> PISPIETVPVKLKPGMDGPKVKQWPLTEEKIKALVEICTEMEKEGKISKIGPENPYNTPVFAIKKKDSTKWRKLVDFRELNKRTQDFWEVQLGIPHPAGLKKNKSVTVLDVGDAYFSVPLDEDFRKYTAFTIPSINNETPGIRYQYNVLPQGWKGSPAIFQSSM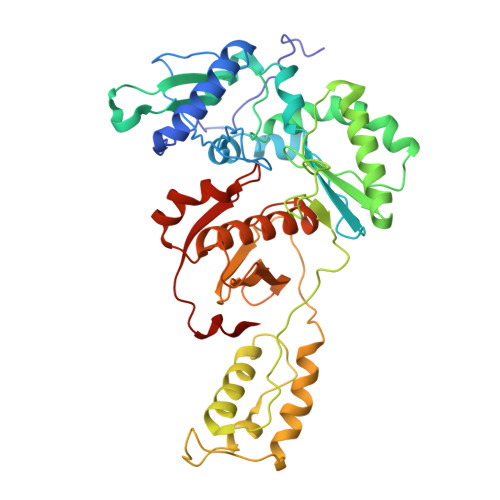TKILEPFKKQNPDIVIYQYMDDLYVGSDLEIGQHRTKIEELRQHLLRWGLTTPDKKHQKEPPFLWMGYELHPDKWTVQPIVLPEKDSWTVNDIQKLVGKLNWASQIYPGIKVRQLSKLLRGTKALTEVIPLTEEAELELAENREILKEPVHGVYYDPSKDLIAEIQKQGQGQWTYQIYQEPFKNLKTGKYARMRGAHTNDVKQLTEAVQKITTESIVIWGKTPKFKLPIQKETWETWWTEYWQATWIPEWEFVNTPPLVKLWYQLE>MTDQNLPVTVAGLGPMGSALAAALLDRGHDVTVWNRSPGKAAPLVAKGARQADDIVDAVSASRLLVVCLADYDALYSALGPAREALRGRVVVNLNSGTPKEANEALRWAERHGTGYLDGAIMVPPAMVGHPGSVFL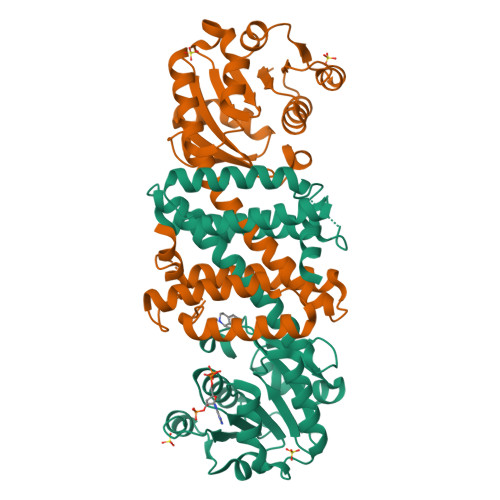YSGSAEVFEEYKETLAGLGDPVHLGTEAGLAVLYNTALLSMMYSSMNGFLHAAALVGSAGVPAAEFTKLAVDWFLPAVIGQIIKAEAPTIDEGVYPGDAGSLEMNVTTLKHIIGTSQEQGVDTEIPVRNKELLDRAVAAGFGESSYYSVIELWR[2x]>MGPSLDFALSLLRRNIRQVQTDQGHFTMLGVRDRLAVLPRHSQPGKTIWIEHKLVNVLDAVELVDEQGVNLELTLITLDTNEKFRDITKFIPENISTASDATLVINTEHMPSMFVPVGDVVQYGFLNLSGKPTHRTMMYNFPTKAGQCGGVVTSVGKVIGIHIGGNGRQGFCAGLKRSYFASE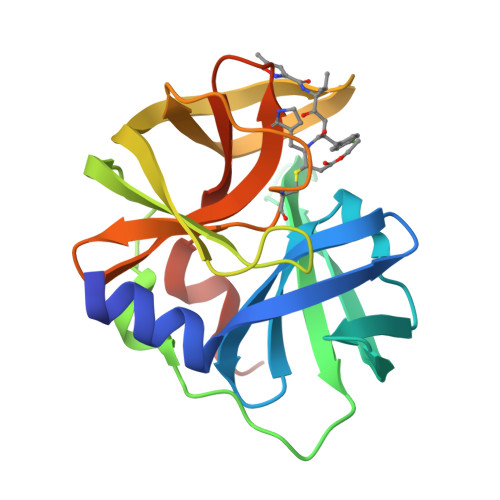QHHHHHH[8x]> DAASVYTLPAGADFLMCYSVAEGYYSHRETVNGSWYIQDLCEMLGKYGSSLEFTELLTLVNRKVSQRRVDFCKDPSAIGKK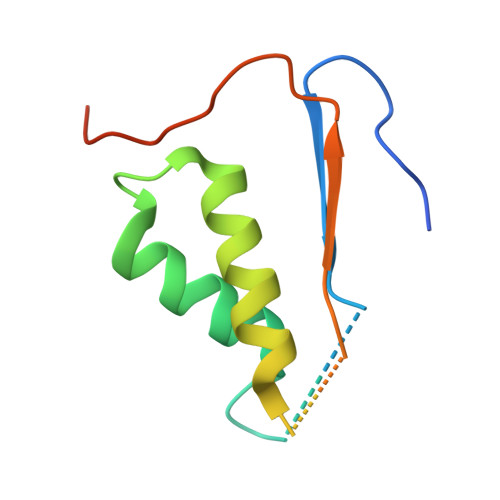QVPCFASMLTKKLHFFPKSNRHHHHHH> MNKPVIEGYKVSGYILPDFSFDATVAPLVKAGFKVEIVGTELYAVTDANGYFEITGVPANASGYTLKISRATYLDRVIANVVVTGDTSV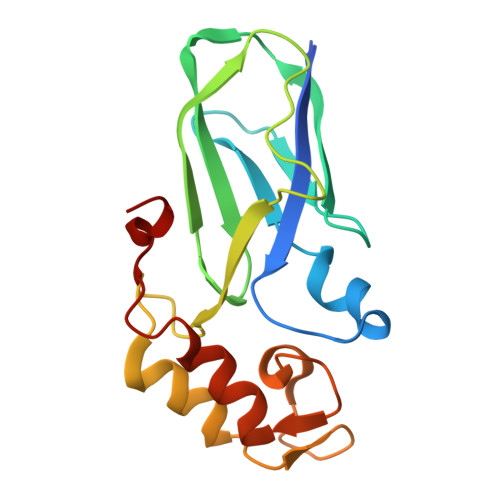STSQAPIMMWVGKIVKDNSINLLDVAEVIRCFNATKGSANYVEELDINRNGAINMQDIMIVHKHFGATSSDYDAQ>[2x]SLLNVPAGKDLPEDIYVVIEIPANADPIKYEIDKESGALFVDRFMSTAMFYPCNYGYINHTLSLDGDPVDVLVPTPYPLQPGSVTRCRPVGVLKMTDEAGEDAKLV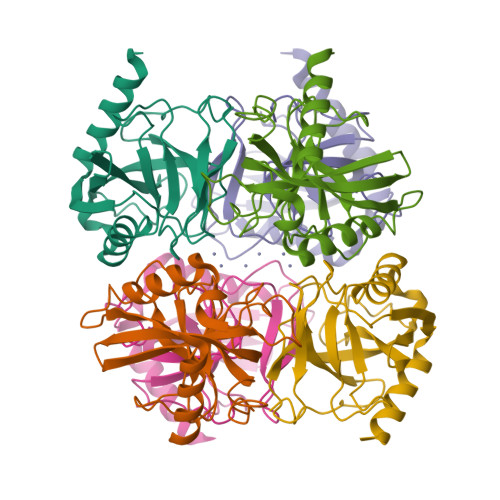AVPHSKLSKEYDHIKDVNDLPELLKAQIAHFFEHYKDLEKGKWVKVEGWENAEAAKAEIVASFERAKNK>[3x]XMFIVNTNVPRASVPDGFLSELTQQLAQATGKPPQYIAVHVVPDQLMAFGGSSEPCALCSLHSIGKIGGAQNRSYSKLLCGLLAERLRISPDRVYINYYDMNAANVGWNNSTFA

Macrophage migration inhibitory factor (MIF) is expressed at high levels in various inflammatory diseases and cancer. Macrophage migration inhibitory factor promotes directional cell migration (or chemotaxis) of various cell types 2, 3, 4. Unlike canonical cytokines and chemokines, a trimeric MIF molecule has three tautomerase active sites at the trimer interfaces 23. Although the enzymatic activity is vestigial, there is accumulating evidence that the active site is important for receptor binding 24, 25.

To structurally verify the proposal for the inhibition of p110γ and p101 expression, we co‐crystallized 1, 2 and 12 with MIF. 1 occupies the bottom half of the catalytic pocket, whereas 2 occupies the upper half. However, this steric hindrance theory does not explain the inhibition of MIF‐induced migration of THP‐1 cells and HL60 cells by 1 that does not have any solvent‐exposed ring structure like 2. In contrast, MIF:ISO‐1, MIF:1 and MIF:2 show relatively increased B‐factors (>10 Å2, >30 Å2, and >25 Å2 respectively) for the L2 loop. As MIF:1, MIF:2 and MIF:ISO‐1 inhibited MIF‐induced leucocyte migration and increased B‐factors in L2, it is likely that structural stability of L2 is the critical structural determinant for the chemoattractant activity of MIF. Pro1 attached to 1 revealed the longest displacement (1.9 Å) followed by 4‐IPP (1.1 Å), 2 (0.8 Å), 12 (0.5 Å) and ISO‐1 (0.4 Å). This suggests that 1 might disturb the protein the most. The displacements are 1.1 Å for 1, 0.6 Å for 4‐IPP, 0.6 Å for 2 and 0.5 Å for ISO‐1 and 0.2 Å for 12. This suggests that the displacement of Pro1 upon inhibitor binding within the tight active site pushes and destabilizes the L2 loop, resulting in suboptimal MIF binding to receptor. 1 inhibited 79% of the total number of neutrophils otherwise recruited by MIF.>MPSPVTTFGPKATVETQDPASVRLTWNKSPKSVLVIKKMRDASLLQPFKELCTHLMEENMIVYVEKKVLEDPAIASDESFGAVKKKFTTFREDYDDISNQIDFIICLGGDGTLLYASSLFQGSVPPVMAFHLGSLGFLTPFSFENFQSQVTQVIEGNAAVVLRSRLKVRVVKELRGKKTAVHNGLGENGSQAAGLDMDVGKQAMQYQVLNEVVIDRGPSSYLSNVDVYLDGHLITTVQGDGVIVSTPTGSTAYAAAAGASMIHPNVPAIMITPICPHSLSFRPIVVPAGVELKIMLSPE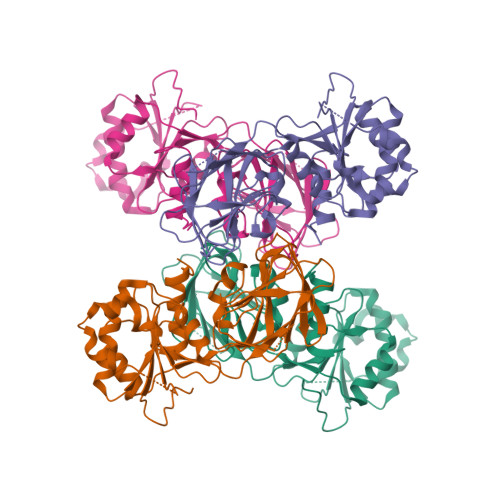ARNTAWVSFDGRKRQEIRHGDSISITTSTYPLPSICVRDPVSDWFESLAQCLHWNVRKKQAHFELGLEHHHHHH[4x]> MELHQIRGCHKNDIELKKYNIGVAISLGNKWFSIDNIEKLVKWSLLHTKEYVIIYIADSIHGINLSVRNKLSDSHAEEVAIRYGRNLFIKIKE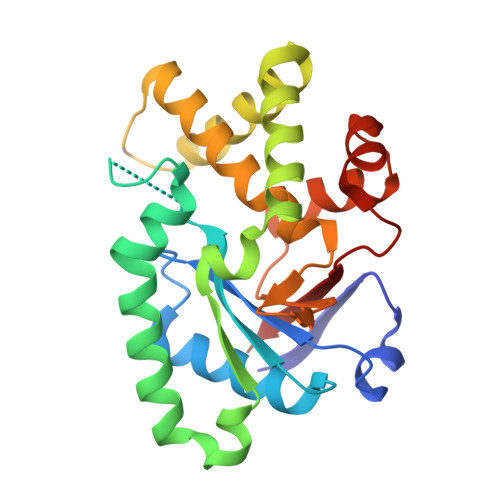RVSLSFSQDEQAKIIYATWSDIADSKYKEKVKYLYNLYDKNINFKNYIENFVKEWVSKEKRTFNNNEINKFGRYILEELPELMVQVKARGVLFEAYVYPYKTRITEFVGLLQKGEIFPEIKTNILDNHPKIFLEVRE>UUGCGUCCCGUCGACGAAGUCGC[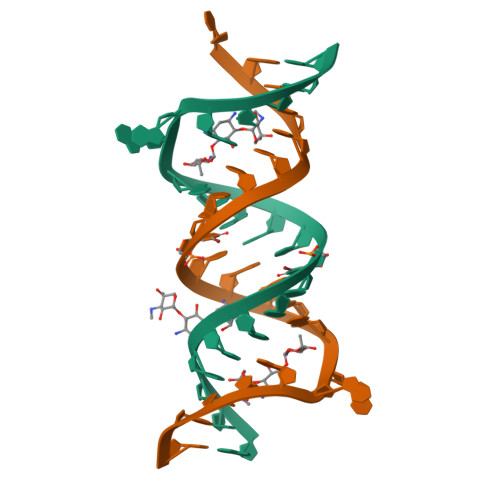2x]>[14x]AEPVYPDQLRLFSLGQGVCGDKYRPVNREEAQSVKSNIVGMMGQWQISGLANGWVIMGPGYNGEIKPGTASNTWCYPTNPVTGEIPTLSALDIPDGDEVDVQWRLVHDSANFIKPTSYLAHYLGYAWVGGNHSQYVGEDMDVTRDGDGWVIRGNNDGGCDGYRCGDKTAIKVSNFAYNLDPDSFKHGDVTQSDRQLVKTVVGW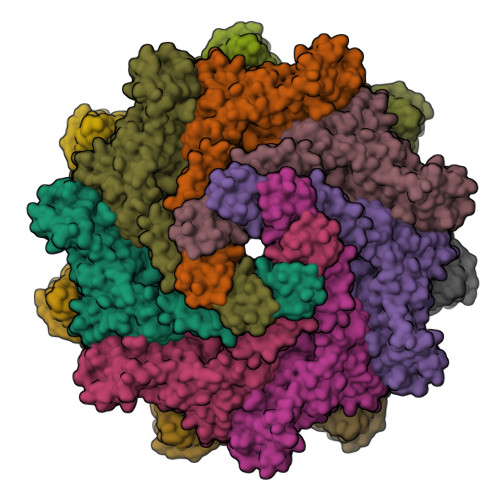AVNDSDTPQSGYDVTLRYDTATNWSKTNTYGLSEKVTTKNKFCWPLVGETELSICIAANQSWASQNGGSTTTSLSQSVRPTVPARSKIPVKIELYKADISYPYEFKADVSYDLTLSGFLRWGGNAWYTHPDNRPNWNHTFVIGPYKDKASSIRYQWDKRYIPGEVKWWDWNWTIQQNGLSTMQNNLARVLRPVRAGITGDFSAESQFAGNIEIGAPVPLAA> VFFWSE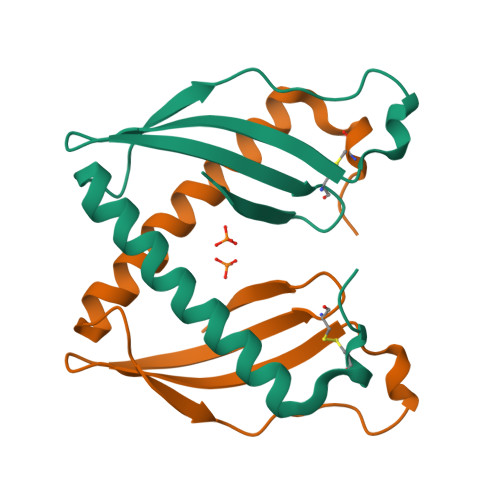DKGPACYQVSDEQARTFVKNDYLQRMKRWDNDVQLLGTEIPKITWEKIERSLTDVEDEKTLLVPFKAEGPDGKRMYYGMYHCEEGYVEYAND> IQINQVRPKLPLLKILHAAGAQG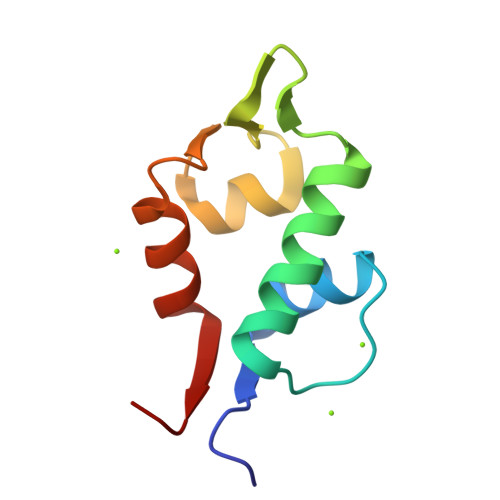EMFTVKEVMHYLGQYIMVKQLYDQQEQHMVYCGGDLLGELLGRQSFSVKDPSPLYDMLRKNLVTLAT;> LTFEHYWAQLTS>[2x]MTMIIRKYFSGIPTIGVL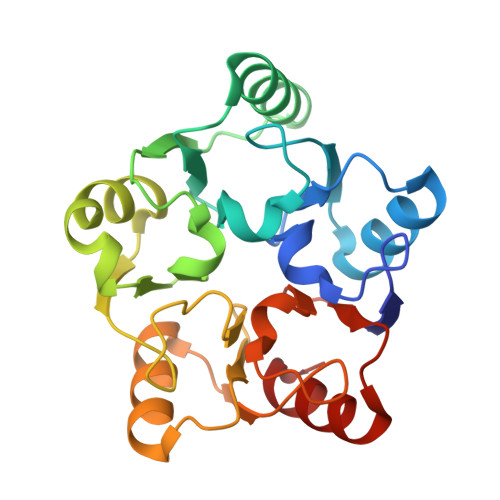ALTTEEITLLPIFLDKDDVNEVSEVLETKCLQTNIGGSSLVGSLSVANKYGLLLPKIVEDEELDRIKNFLKENNLDLNVEIIKSKNTALGNLILTNDKGALISPELKDFKKDIEDSLNVEVEIGTIAELPTVGSNAVVTNKGCLTHPLVEDDELEFLKSLFKVEYIGKGTANKGTTSVGACIIANSKGAVVGGDTTGPELLIIEDALGLI> MALELAVDWRIDNILEAIILMLPAMIANATPVVAGGRRPVDMGVVLPDGRRL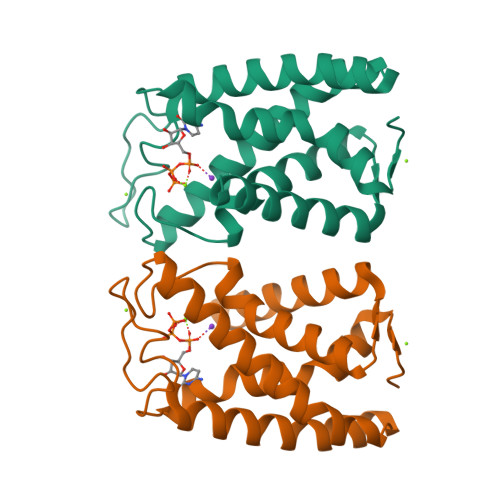LGDGKTIEGLLAGFAAGSAAGVLAALASGNMLLAVHSPAIALGALAGDMAGSFVKRRLGIERGRPAPLLDQLDFYLGALAVSIALGYTWTPRVAVEAAAAVLLLHLAANITAYLLGLKKVPWLEHHHHHH>[2x]MSATKSIVGEALEYVNIGLSHFLALPLAQRISLIIIIPFIYNIVWQLLYSLRKDRPPLVFYWIPWVGSAVVYGMKPYEFFEECQKKYGDIFSFVLLGRVMTVYLGPKGHEFVFNAKLADVSAEAAYAHLTTPVFGKGVIYDCPNSRLMEQKKFVKGALTKEAFKSYVPLIAEEVYKYFRDSKNFRLNERTTGTIDVMVTQPEMTIFTASRSLLGKEMRAKLDTDFAYLYSDLDKGFTPINFVFPNLPLEHYRKRDHAQKAISGTYMSLIKERRKNNDIQDR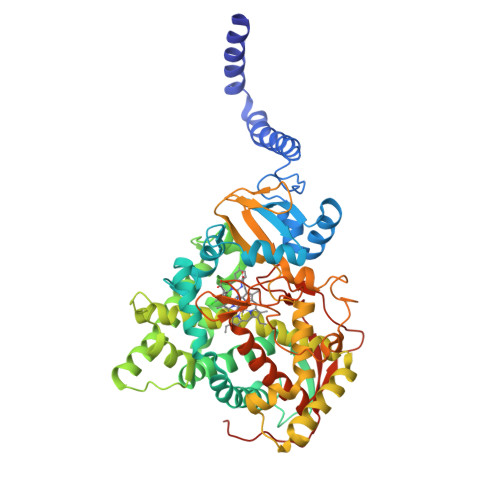DLIDSLMKNSTYKDGVKMTDQEIANLLIGVLMGGQHTSAATSAWILLHLAERPDVQQELYEEQMRVLDGGKKELTYDLLQEMPLLNQTIKETLRMHHPLHSLFRKVMKDMHVPNTSYAIPAGYHVLVSPGYTHLRDEYFPNAHQFNIHRWNNDSASSYSVGEEVDYGFGAISKGVSSPYLPFGGGRHRCIGEHFAYCQLGVLMSIFIRTLKWHYPEGKTVPPPDFTSMVTLPTGPAKIIWEKRNPEQKIGGRHHHHHH> MADNTKPNRMPVAPYWTSPEKMEKKLHAVPAAKTVKFKCPSSGTPQPTLRWLKNGKEFKPDHRI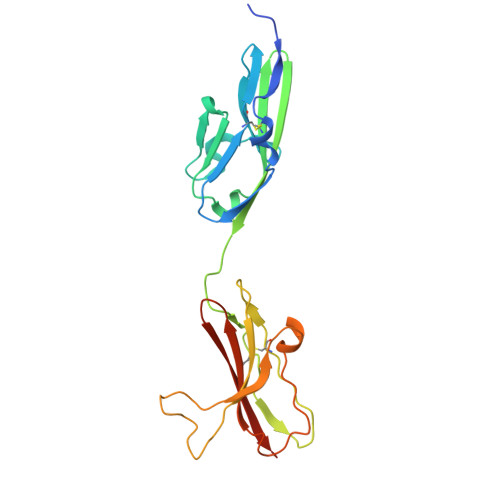GGYKVRYATWSIIMDSVVPSDKGNYTCIVENEYGSINHTYQLDVVERSPHRPILQAGLPANKTVALGSNVEFMCKVYSDPQPHIQWLKHIEVNGSKIGPDNLPYVQILKTAGVNTTDKEMEVLHLRNVSFEDAGEYTCLAGNSIGLSHHSAWLTVLEALEER>[3x]PPGPPGPPGP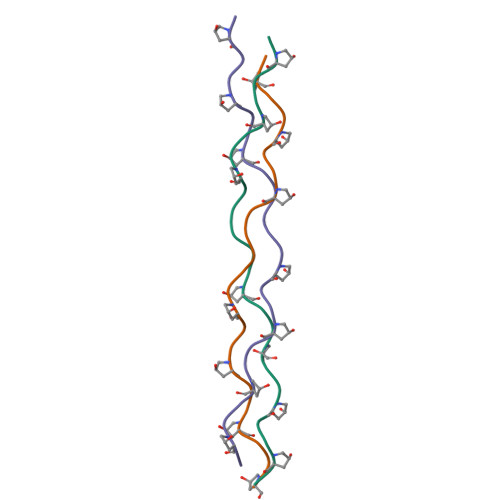RGPPGPPGPPGPPG> MGKRILLLEKERNLAHFLSLELQKEQYRVDLVEEGQKALSMALQTDYDLILLNVNLGDMMAQDFAEKLSRTKPASVIMILDHWEDLQEELEVVQRFAV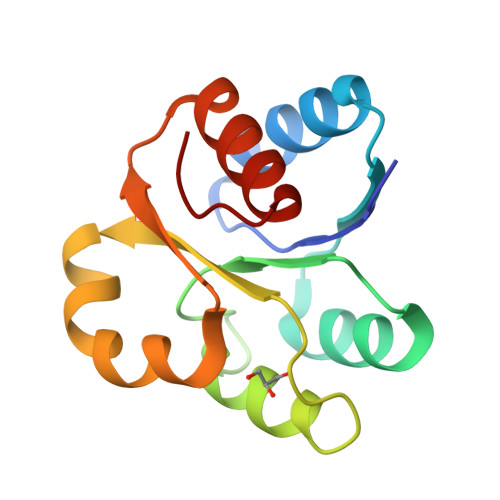SYIYKPVLIENLVARISAIFRGRDFI>MATEFGTAVNHADLVERLVQFLTASPDLVAAGQAYEKVFDNTIPASGTAIAVRQVTLRAPGLGGTDAIYMGIQSYGDTALDYYNLRLMGGTAFNPGAIPPGGDYWTAFANYSPRVQLLAWNQPMPYWFFANGRRFWIVVKVSTIYESAGAGFILPPCPPSQYPYPLAVVGSYRGDVATRWSDVSDRHRGISSPYERSCYLRDPAGRWLGFTVDGGAANESDYNNRTLLPLGCGRYAGSSDTVVKQLRDSFGKFPLKALQFVTRETEGRRYLGDFDGAFYVPTLNSGAEDVIVEDGVDHVVFQTAWRSGNPWLYAIRKD[3x];>MAYFTGTANNPADLLAKVRVHAESLGWVTDRASASEWLCHNADGYWSFNAGANQFQMAGNTGFDNSLAWNAQPGNSVQNNPYSSKGPTVAQLSGGPFTRYHLFATAAYLHLHVEIAAGQFRPVMIGSLNKRGVGYTGGQYVCGSFIYTPGQALTNNWSSHPFDGYHIQYSNSSCMLRLDGLDGGPSPEWLPFDYTTNVPRRVVGPGRGNYSSQYHPDVGLIDASANELNSSTTTVPCAIYAFGAQQRSRYVGEVPDFGICNMAFLAPGDPLVVGSDTWRVYPLLQRGTATDFDSTSAWVGYCFRVVE[3x]

Bacteriophage Casadabanvirus JBD30, from the order Caudoviricetes, is a temperate phage that infects the bacterium Pseudomonas aeruginosa. The virion of bacteriophage JBD30 is composed of an icosahedral capsid, long flexible non-contractile tail, and a baseplate. Using its baseplate, JBD30 attaches to Pseudomonas aeruginosa via the bacterial type IV pilus, whose subsequent retraction brings the phage to the bacterial cell surface.

Three tail fibres resembling bent arms protrude laterally from the baseplate. Each of the arms is composed of three heterodimers of gp47 and gp48, which are rotated 180° relative to each other. The folds of gp47 and gp48 are similar. Gp47 was classified as a hydrolyse belonging to a nitrilase superfamily of proteins. In contrast, gp48 could not be classified into any enzyme family. A loop and three-stranded β-sheets of gp47 form a positively charged surface depression, which binds the negatively charged α-helix of gp48. The gp48 fold is stabilized by a disulfide bond between Cys142 and Cys174. Bacteriophage JBD30 uses its baseplate tail fibre to bind the pilus. The arrangement of the three heterodimers of proteins gp47 and gp48 is such that they form a unique interface, which can embrace the pilus. Side chains of pilA residues Lys68 and Lys112 are predicted to interact with Asp185 of gp47 and Tyr169 of gp48, respectively.>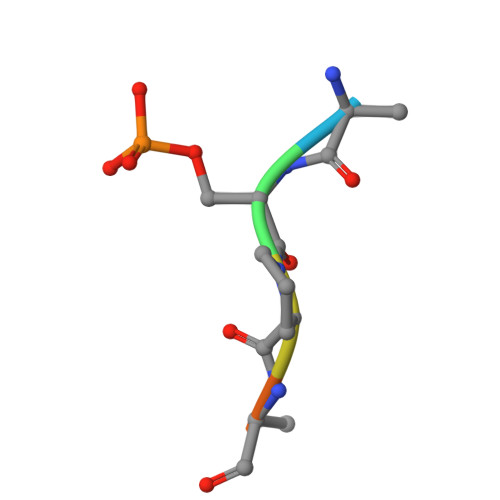 ASPRRR4-(4-chlorophenyl)-1-[(3S)-3,4-dihydroxybutyl]-N-[3-(4-methylpiperazin-1-yl)propyl]-3-phenyl-1H-pyrrole-2-carboxamide | C29 H37 Cl N4 O3 | 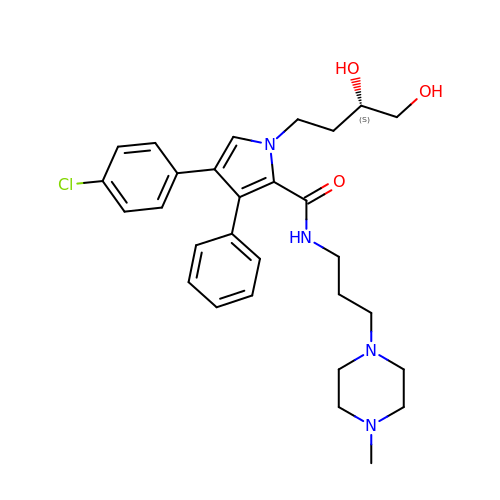DXJMWRCEEVNUJU-VWLOTQADSA-N> MDIQRVKRLLSITNDKHDEYLTEMVPLLVEFAKDECHNPFI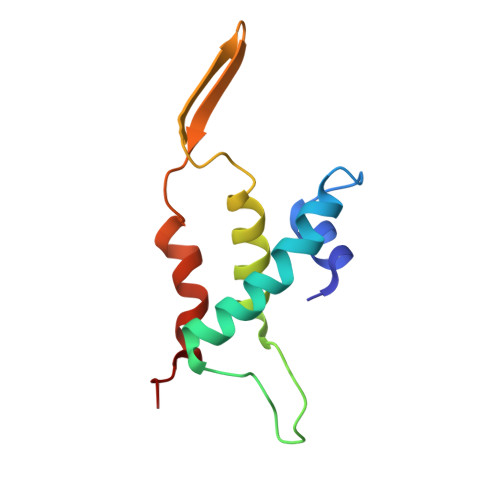DKDGNESIPSGVLIFVAKAAQFYMTNAGLTGRSMDTVSYNFATEIPSTILKKLNPYRKMAR(1S)-1,5-anhydro-1-(3-chloro-2,5-dihydroxyphenyl)-D-glucitol 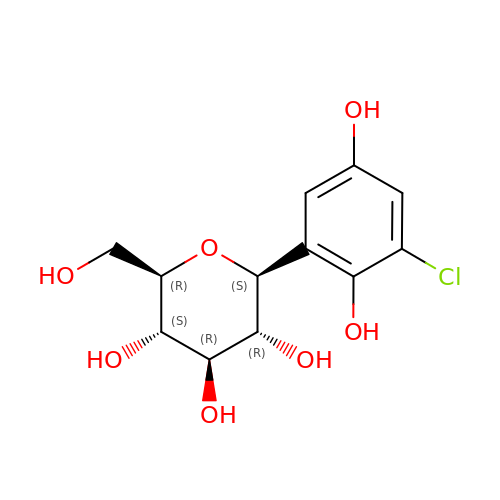| C12 H15 Cl O7 | SCGLZDHCPHCUAO-URYVQPGZSA-N> SAPAPPSGWSQVFLDDFDGAAGSSVNTANWQFDTGTSYPGGAGNWGTGEVESMTSSTSNVSLDGNGDLLITPRRDASGNWTSGRIETTRTDFQPPAGGKLR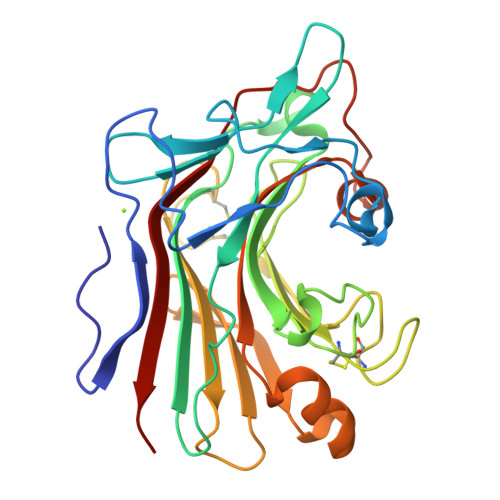VEARLQMPNVTGDAAAGYWPAFWMLGAPFRGNYQNWPGVGELDIMENVQGLNKTWATMHCGTSPGGPCNETSGIGNSTACPNTTCQSGFHTYTMEWDRSVSPEAIRFSVDGVTYQTVTANQMDAATWTNATNHGFFVILNVAMGGGFPGAFGGGPTGATEPGHPMVVDYVQVTSLSPGL Family VIII esterases present similarities to class C β‐lactamases, which show nucleophilic serines located at the S‐X‐X‐K motif instead of the G‐X‐S‐X‐G or G‐D‐S‐(L) motif shown by other carboxylesterase families. Indeed, the analysis of the substrate specificity revealed its capacity to hydrolyse nitrocefin as a model chromogenic cephalosporin substrate (40.4 ± 11.4 units·g−1), and a large battery of 66 structurally different esters (up to 1730 min−1), including bis(2‐hydroxyethyl)‐terephthalate (241.7 ± 8.5 units·g−1) and the mycotoxin T‐2 (1220 ± 52 units·g−1). It also showed acyltransferase activity through the synthesis of benzyl 3‐oxobutanoate (40.4 ± 11.4 units·g−1) from benzyl alcohol and vinyl acetoacetate.

Structural analyses of free and substrate‐bound forms of this homooctamer esterase suggest that EH7 presents a more opened and exposed S1 site having no steric hindrance for the entrance of substrates to the active site, more flexible R1, R2 and R3 regions allowing for the binding of a wide spectrum of substrates into the active site, and small residues in the conserved motif Y‐X‐X containing the catalytic Tyr enabling the entrance of large substrates. These unique structural elements in combination with docking experiments allowed us to gain valuable insights into the substrate specificity of this esterase and possible others belonging to family VIII.

>[8x]MHHHHHHHHHHLEVLFQGPSEFPMAQSNIIAGMDLNRLDRIAEHLDRAYLHPGKLAGTMTLVARRGEVVYCQAQGLRDVERQLPVERDTLFRIYSMTKPITSIALMQLYEQGRFLLDEPVHKYIPTWKNLRVYKTGSHPQMLTTAPQRPMTIRDLLTHQSGLTYGFMNRTNVDAAYRSLKLDGGPGHTLDRLIDELARLPLEFSPGTAWNYSVATDVCGYLVQLLSGMSLDDYFSKHIFQPLGMPDTFFTVPAEKLSRFAACYEYQPGDSFSLQDDPQGSAFAKAHGYLSGGGGLVSCVDDYYRFAQALANGGELDGARIIGRKTLEFMRMNHLPDNKGLPDVAIGSFSETPYDGTGFGLGFSVKLDVAKSQTVGSVGEYGWGGMASTNFFIDPEEDLLMVFMTQLIPSSTYAVRQELRAIINGALVDA> MIFRNRVVDKGQLRNLISWAFTHYGTARTAVMADKLKDLGFRYATRAGVSISVDDLMVPPSKRSLLEAAEEEIRATEVRYQRGEITEVERFQKVIDTWNGTSEALKDEVVTHFKQTNPLNSVYMMAFSGA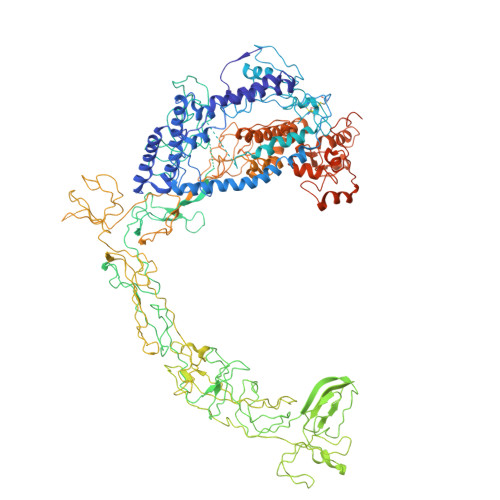RGNISQVRQLVGMRGLMADPQGEIIDLPIKTNFREGLTVTEYIISSYGARKGLVDTALRTADSGYLTRRLVDVSQDVIIREIDCGTTRGIPVRPMTEGSKTLIKLSTRLLGRVVGEDVIHPKTKEVIAPRNTPISDDLAKEIEKAGVAEVVVRSPLTCEAARSVCQHCYGWSLAHAKMVDLGEAVGIIAAQSIGEPGTQLTMRTFHTGGVFTGEVAQQVRSKMDGTIKLPRKLRTRTHRTRHGEDALFVESNGIMILEPRKEGSETPAPQEIHVTQGSTIYIVDGQQVKKGQLLAEVALGGRTTRTNTEKAVKDVASDLAGEVKFAEVVPEQKTDRQGNTTTTAARGGLIWILSGEVYNLPPGAELVVKNGDRVETNGVLAETKLTTIHGGVVRLPEATPGKSTREIEIITASVVLDQATVTVQSSQGRNNYLITTGNNQVFNLRATPGTKVQNGQVVAELIDDRYRTTTGGFLKFAGVEVQKKGKAKLGYEVVQGGTLLWIPEETHEVNKDISLLLVEDGQYVEAGTEVVKDIFCQNSGVVEVTQKNDILREVVVKPGELLMVDDPEAVIGRDNTLLQPGEELLGQVATELRYIQYVESPEGPALLSRPVVEFAVPSNPDVPSTTSVSQQTGRSIQMRAVQRLPYKDSERVKSVEGVELLRTQLVLEIEQEGEQEHNASPLAADIELIPDLEDADVQRLQLVILESLVLRRDIAADATQGSTQTSLEVKDGDTIVPGSVVARTQILSKEGGIVRGVQKGSEAVRRCLVLRHSDMATLNISAKPKVKAGDLIVAGTELAPGIFAEESGQIVGVKNAGESTTTQDAALSTQNYAVTIRAGRPYRVSPGAVLQIEDGDLVQRGDNLVLLVFERAKTGDIIQGLPRIEELLEARKPKEACILAKRGGEVKVVYGDGDEAIAIKVIESNGVVTDYPLGPGQNLAMPDGSVVPAGQPLSDGPSNPHEILEVFFSLGSEDGVYACASHALQKVQTFLVNEVQMVYQSQGIDIADKHIEVIVRQMTNKVRIDDGGDTTMLPGELVELRQVEQVNEAMAITGGARAQYTPVLLGITKASLNTDSFISAASFQETTRVLTEAAIEGKSDWLRGLKENVIIGRLIPAGTGYNTYDEPGMLEDYSTLETTSVLDETDDPLDMVLDDRTARAYNLDSPGLAETGFNNRRSILDDDELIADEIHDLVEAEVEVDDEVDDDYEDDDEDDDDYED> GSHMMKGGSRVSNPAVMAQEEEDVRDYNLTEEQKAIKAKYPPVNRKYEYLDHTADVQLHAWGDTLEEAFEQCAMAMFG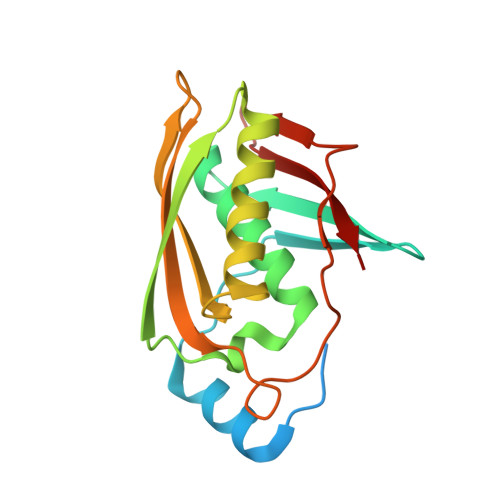YMTDTGTVEPLQTVEVETQGDDLQSLLFHFLDEWLYKFSADEFFIPREVKVLSIDQRNFKLRSIGWGEEFSLSKHPQGTEVKAITYSAMQVYNEENPEVFVIIDI methyl 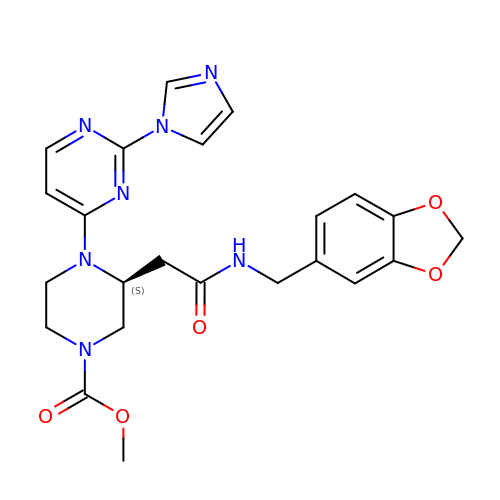(3S)-3-{2-[(1,3-benzodioxol-5-ylmethyl)amino]-2-oxoethyl}-4-[2-(1H-imidazol-1-yl)pyrimidin-4-yl]piperazine-1-carboxylate | C23 H25 N7 O5 | NVYMEDQKBQMAKF-KRWDZBQOSA-N> GPMDLYSTPAAALDRFVARKLQPRKEFVEKARRALG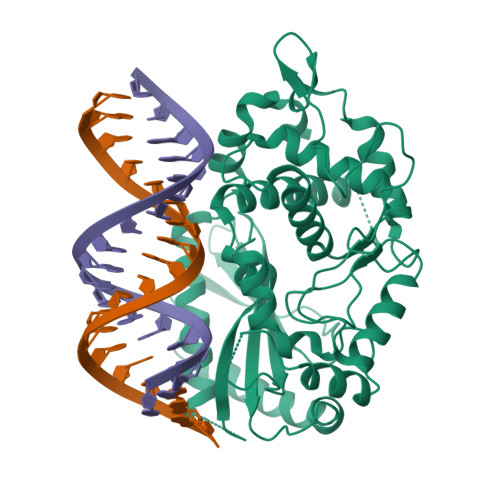ALAAALRERGGRLGAAAPRVLKTVKGGSSGRGTALKGGCDSELVIFLDCFKSYVDQRARRAEILSEMRASLESWWQNPVPGLRLTFPEQSVPGALQFRLTSVDLEDWMDVSLVPAFNVLGQAGSGVKPKPQVYSTLLNSGCQGGEHAACFTELRRNFVNIRPAKLKNLILLVKHWYHQVCLQGLWKETLPPVYALELLTIFAWEQGCKKDAFSLAEGLRTVLGLIQQHQHLCVFWTVNYGFEDPAVGQFLQRQLKRPRPVILDPADPTWDLGNGAAWHWDLLAQEAASCYDHPCFLRGMGDPVQSWKGPGLPRAGCSGLGHPIQLDPNQKTPENSKS>[2x]MGHHHHHHGNITLTKRQQEFLLLNGWLQLQCGHAERACILLDALLTLNPEHLAGRRCRLVALL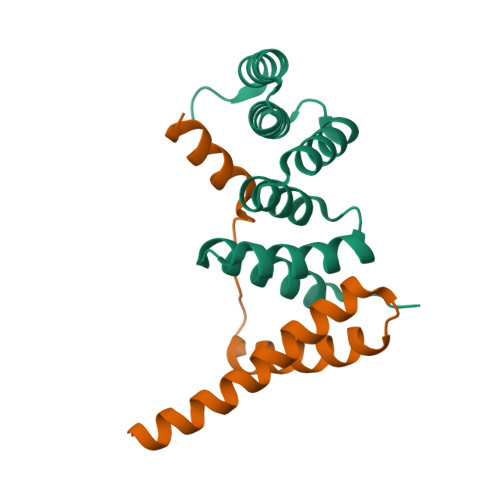NNNQGERAEKEAQWLISHDPLQAGNWLCLSRAQQLNGDLDKARHAYQHYLELKDHNESP;>GAMGTAQSKRSLWDFASPGYTFHGLHRAQDYRRELDTLQSLLTTSQSSELQAAAALLKCQQDDDRLLQIILNLLHKV[2x]> MAPSAEGASGAPTPEDLKLHQLSQKYTAEAAKRFRPEGLGQFIRLKEVGNERFRALAEDPWVDHAALNAKEPVKDGSRYKFIILGAGYGGLLYAVRLAEAGLASGPDDILMVDAAGGFGGTWWWNRYPGLHCDVESYSYMPLLEETGYIPKSKYAAGPELLEHAYRIATQWKLHDKALFRSNVKTIRWDDESRLWSLEVTEGRGPGQQSRELKLQARYVLLASGILTNPQVPKIPGLETFTGPVFHTARWNYDVTGGSPTDEALNRLEGKRVGIIGTGATAIQVVPKLAKYAKELYVFQRTPSGVWWRGQRPTDPVEWKTKIARKKGWQRERMLNLDSYLTDAAEEGQENMVADGWTEMPAFSAVIGSPRHGIVEPTPEKIAEHLGRLYKLDLPHAEQVRARTDSIVKDPKTAAKLKAWYP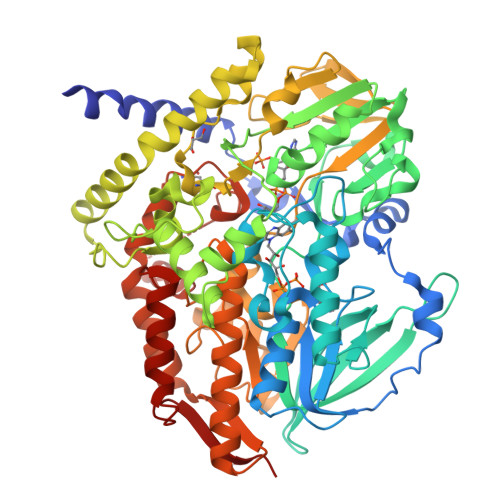TWCKRPTFSDEYLQTFNLPNVHLVDTDGKGVDAANPSGLVVADKEYPLDILVLSTGYVTPSIGGGSPAVRTGVDIYGRGGKSLDDKWQTHGAATLHGVCSNGFPNLFFTPLSQSSQAANNAFTLDVGTEHIVQVIKTAEDRVDGDALVEVTSEAEEAWSFEIMKHAGWFASVTGCTPGYITSEGEALRKSEDPMEMAKRARSGNLSQGMASYMKLLQEYRADGSLKGFDISSRA>[2x]GMLTENPVLQAIRQRRSIRRYTDEAVSDEAVRLILEAGIWAPSGLNNQPCRFLVIRADDPRCDILAAHTRYGHIVRGAKVIILVFLDREAMYNEVKDHQAAGAAVQN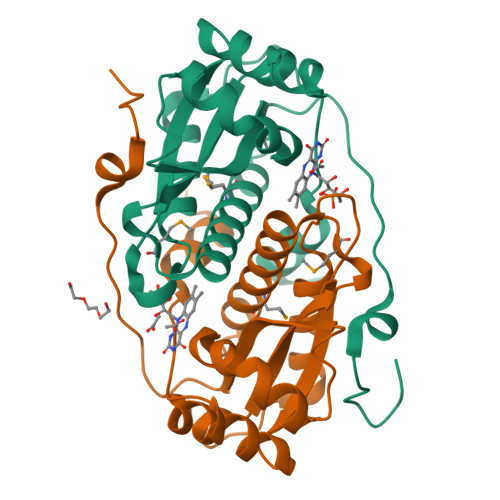MLLAAHALQLGAVWLGEIINQAATLLPALALDPARLSFEAAIAAGHPAQNGSSSRRPLAELLLEEPFPQPE> MGAQMSKNTAGSHTTGTYATGGSNIHYTNINY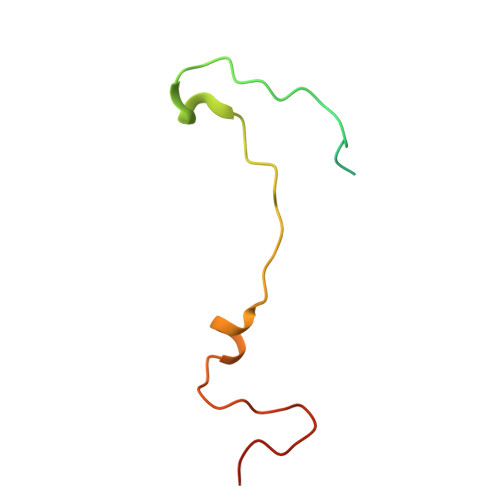YENAASNSLNKQDFTQDPEKFTRPVVDVMKEAAVPLKSP2-[2-(1-CARBAMIMIDOYL-PIPERIDIN-3-YL)-ACETYLAMINO]-3-{4-[2-(3-OXALYL-1H-INDOL-7-YL)ETHYL]-PHENYL}-PROPIONIC ACID 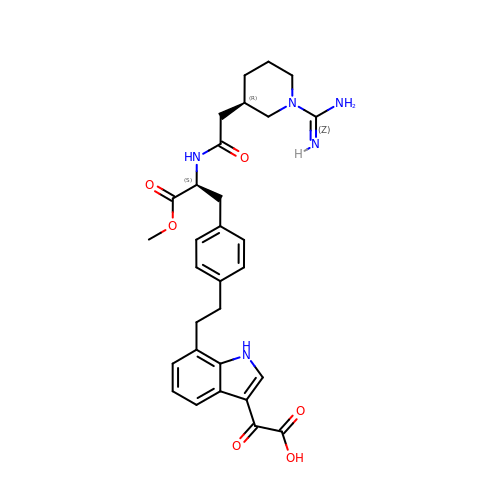METHYL ESTER | C30 H35 N5 O6 | YRVAENMKEUHMEX-YKSBVNFPSA-N> MQDILDFYEEVEKTINPPNYFEWNTYRVF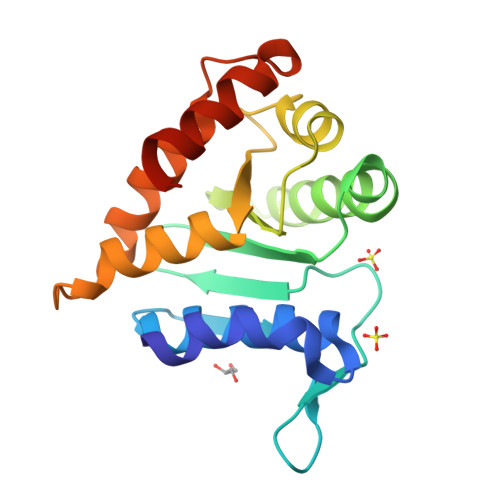KKLGSYKNLVPNFKLDDSGHPIGNAIPGVEDILVEYEHFSILIECSLTIGEKQLDYEGDSVVRHLQEYKKKGIEAYTLFLGKSIDLSFARHIGFNKESEPVIPLTVDQFKKLVTQLKGDGEHFNPNKLKEILIKLLRSDLGYDQAEEWLTFIEYNLKHHHHHH>MESCYNPGLDGIIEYDDFKLNSSIVEPKEPAPETADGPYLVIVEQPKQRGFRFRYGCEGPSHGGLPGASSEKGRKTYPTVKICNYEGPAKIEVDLVTHSDPPRAHAHSLVGKQCSELGICAVSVGPKDMTAQFNNLGVLHVTKKNMMGTMIQKLQRQRLRSRPQGLTEAEQRELEQEAKELKKVMDLSIVRLRFSAFLRASDGSFSLPLKPVISQPIHDSKSPGASNLKISRMDKTAGSVRGGDEVYLLCDKVQKDDI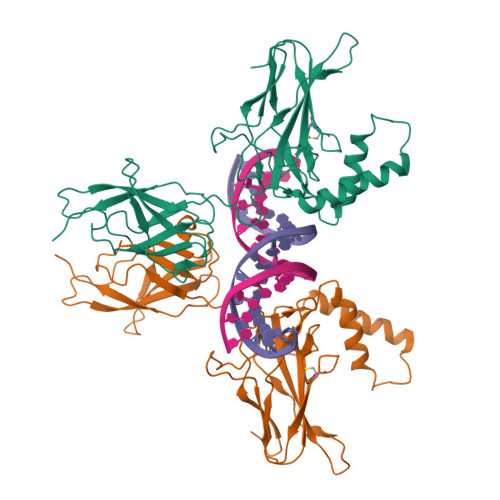EVRFYEDDENGWQAFGDFSPTDVHKQYAIVFRTPPYHKMKIERPVTVFLQLKRKRGGDVSDSKQFTYYPLVEDKEEVQRKRRKALPTFSQPFGGGSHMGGGSGGAAGGYGGAGGGGSLGFFPSSLAYSPYQSGAGPMGCY[2x]>[8x]GSHMVE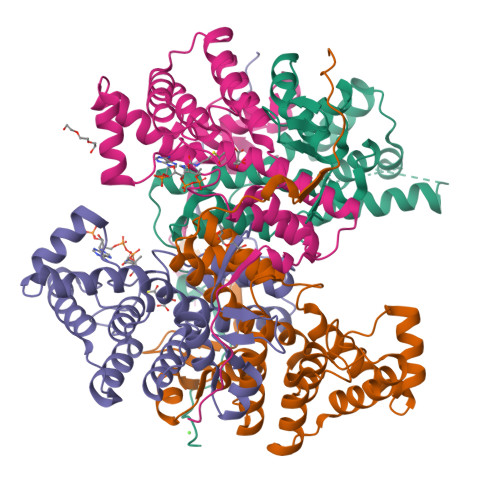PLIRTTISDDRGEEPRYAGYAASELCSKGYGIEDVIGLLWNKKLPTREESEIIKRIVMISADHGPAVSGAFGSILAACAGIDMPQAVSAGMTMIGPRFGGAVTNAGKYFKMAVEDYPNDIPGFLSWMKKNVGPVPGIGHRVKSVKNPDQRVKYLVSYIKNETSLHTPCLDYALEVEKVTTAKKGNLILNVDGTIGCILMDLDFPVHSLNGFFVLARTIGMIGHWIDQNNQNSRLIRLYDYLINYAVKPEQEVPEKK> TPTLQELKTQLEKGNDETKIETMKRILTIMLNGDPLHGLLMHIIRFVMPSKSKPLKKLLYFYYEICPKLDSQGKLKQEFILVCNGIRNDLQHPNEYIRGNTLRFLCKLREPELLEPLLSSVRACLEHRHAYVRKNAVFAVASIYQHAPSLIPDAADLIATFLEGESDPTCKRNGFAALSSISHDKALSYLGTVFEGIPNAEELLQLVEIEFIRKDALHNPQNKPRYLRLIFDLLEANTSTVVYEAASSLTALTNNPVAVKAAAGKFIELAIKEADNNVKL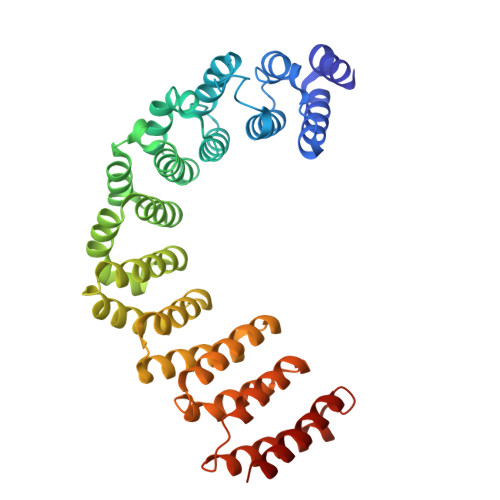IVLDRVDQLRQKNEGILDDLIMEILRVLSSPDIDVRRKALEIALEMVSSKNVEEVVLLLKKELSKTVEQEYEKNSEYRQLLIHSIHQCAVKFS> AMGEVSQWSLKRYGRFMLLDNVGSPGPSSEAAAAGSPTWKVFESSEESGSL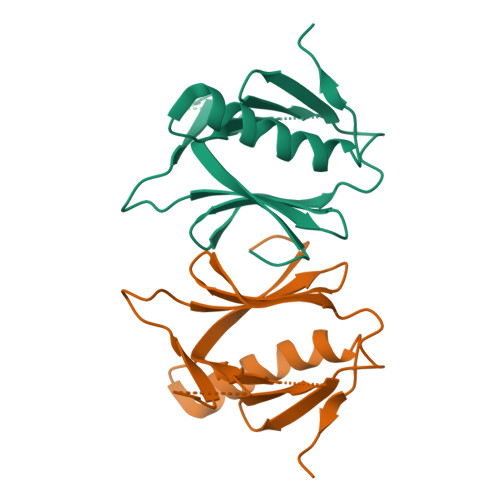VLTIVVSGHFFISQGQTLLEGFSLIGSKNWLKIVRRMDCLLFGTTIKNKSRMFRVQFSGESKEEALERCCGCVQTLAQYVTVQEPDSTTQELQQSQ>[2x]IHMQNPVFSIRLKQAPLVPTLQQLALAHNTNLIIDDELQGTVSLQLENVD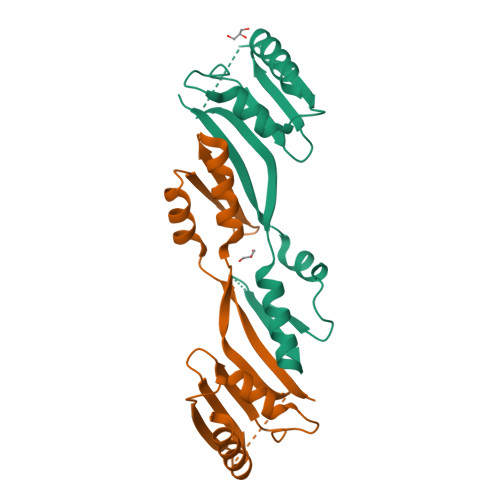LDQLFRSVAKIKQLDLWQENGIYYFTKGDTNTKFAGKMEEPFPLSLPMAEEPAQLNTATIKLHFAKASEVMKSLTGGSGSLLSPNGSITFDDRSNLLLIQDEPRSVRNIKKLIKELDKPIEQLEY>MSSRVPILKVDD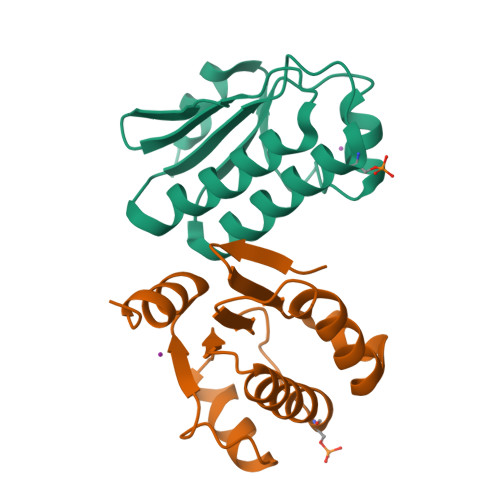YWVVAIEETLHDQSVIQFKEELLHNITGVAGKGLVIDISALEVVDSFVTRVLIEISRLAELLGLPFVLTGIKPAVAITLTEMGLDLRGMATALNLQKGLDKLKNLARMEQR[2x]>[6x]AAESGARSVCNTVRRRSAGMLRKDSQDASDEKYVRGCYFTNW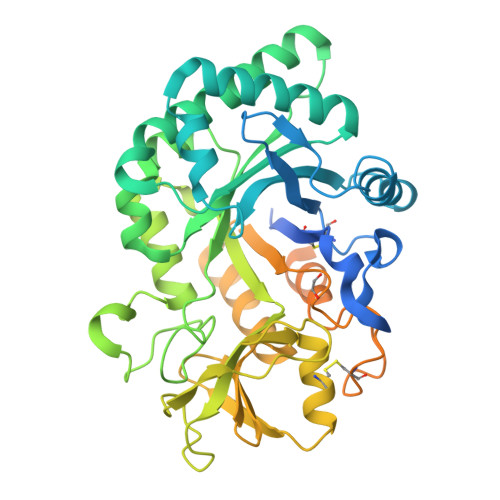AQYRPGNGKYNPEHYQANLCEYIFYAFAKLNDDFTVDQFEWNDIDVLYPGVMKQKSSQPDLKVLLSLGGWNAGTATFKKMAATYSNRAKFISSLVSFLQQNKFDGFDLDWEYPESSDKENYLLLCQEILAKFEEVAKCTSTSRLLFTAAVSANPKTVDAGYDVPALAKVLDFVNLMCYDFHGAWETQTGINSPLYSRKEDSSEFKMWNVEQSSKYWSDKGMPKKQIIIGLPTYGRGWTLSDASKTDIGAPAQGSSTATEYLREAGVISYYEVCQKLSSGAKRVWDDESKTPYLVQGNQWFSYDDVESMKAKINWIKQENYGGAFVWTLDYDDFLGSFCTEHNGKKYPLISLMQEILGGGYVPPSTESTTSQVTTTPSTTTSTTSPAGAFQCPSDGLFPDPESCSNFYQCAGGTAYKMKCPTGLMFNPKTSTCDYPSNVDCQEKTITTHHHHHH> MARIR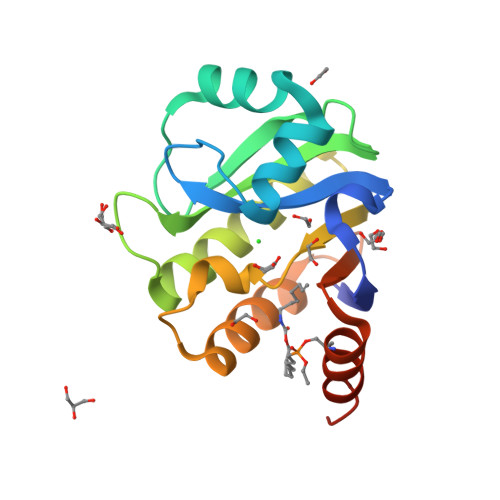HVQGDITEFQGDAIVNAANNYLKLGAGVAGAILRKGGPSIQEECDRIGKIRVGEAAVTGAGNLPVRYVIHAAVLGDEPASLETVRKATKSALEKAVELGLKTVAFTSWGAWVGGLPAEAVHRVMGEEIKKAPDTLEVTGVHGTEKSAEAYRRASLEHHHHHH1-O-phosphono-beta-D-fructofuranose | C6 H13 O9 P 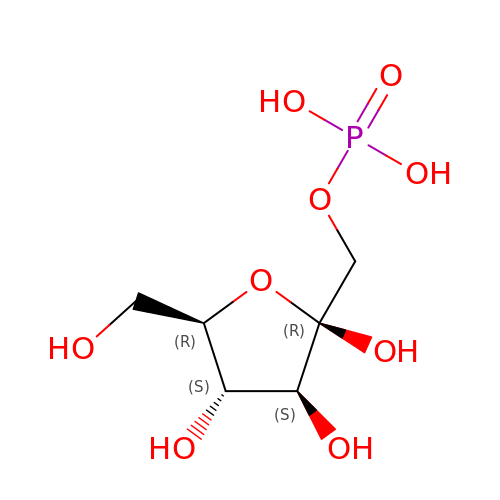| RHKKZBWRNHGJEZ-ARQDHWQXSA-N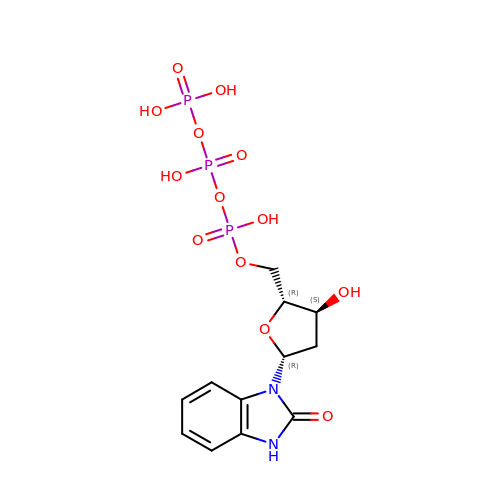[(2~{R},3~{S},5~{R})-3-oxidanyl-5-(2-oxidanylidene-3~{H}-benzimidazol-1-yl)oxolan-2-yl]methyl [oxidanyl(phosphonooxy)phosphoryl] hydrogen phosphate | C12 H17 N2 O13 P3 | OMCWLYQAPHJDBD-HBNTYKKESA-N> GSMSKKPTAGPALHKVIMVGSGGVGKSALTLQFMYDEFVEDYEPTKADSYRKKVVLDGEEVQIDILDTAGQEDYAAIRDNYFRSGEGFLCVFSITDDESFQATQEFREQILRVKNDESIPFLLVGNKCDLNDKRKVPLSECQLRAQQWAVPYVETSAKTRENVDKVFFDLMREIRSRKTEDSKATSGRAKDRCKKRRL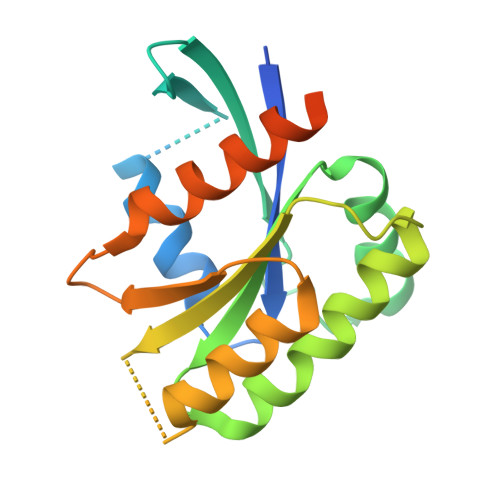KCTLL> MTDRPDHIDSRVWELSETQEDWITQVHGHVRRVVECWKYTICCLISNMHTHRGAPQYDVFKWQDRSTIEWICSKKKVQYPERDTPDLYDNERAVAYKVLLVSDLSDHSPTSGIYHDLAFNLEGEAEESCALVLRGSQLQDIK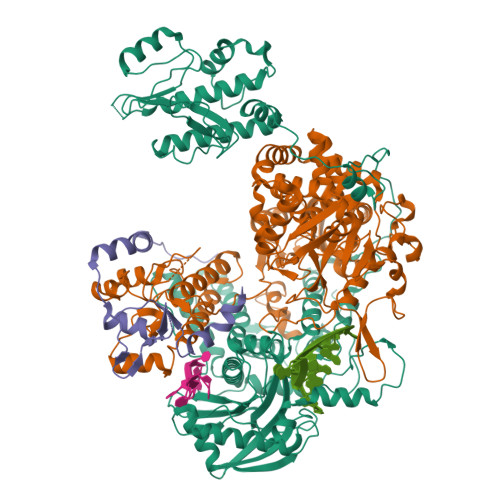GFLCRALEWVVSNNLTQEVVETISGEAKLQFSVGTTFRTLLKRDTDWDVIPTPRVEPNVPRIEGRRWTQMKKLPLLKEKEGPPSPWRALLLGADSEYIVCPPGTDQEAISWIHSQSEIECIRESKSTPASVITCLTSSLQSFAEGNPVRSRIHEDIIAFGINKKQEKKQSASSSASGEWKRAEYQVEEMSLPPWVEEEMVLLRSDQEDNWIELEKNAIYTEVDGVAEGLVDKYIEIVGRTKVASVIEKWQIAATRTFSQLHTDRSRITACPIITRDPSGNCQFWGMVLLGPHHVKRDTDNAPLLIAEIMGEDTEEKYPKHSVFSLKVEGKQFLLSLKITSFSRNKLYTFSNIRRVLIQPASIYSQVVLSRAAENNSLNLEVNPEIQLYLEGAQRGMTLYQWVRMILCLEFLMAIYNNPQMEGFLANMRRLHMSRHAMMERRQVFLPFGSRPEDKVNECIINNPIVAYLAKGWNSMPNVYY;> MNLFTPRSEINPTTTQELLYAYTGPAPVAYGTRTRAVLENIIRPYQYFYKEPNVQRALDIKTGCKEPEDINVEGPSSGFHTASVLKLADNFFRKYRPAMEKLKYWILVKLPKLKYAELSKGRQTYSFIHKRNLPAPIALEETVEFLEQNLRRKIGPTLLSYCQAIADVMELDETTYEGARDPRPWDIQLEEIDSDEEDPLFRQVGREETYTIKFSREELWDQMRTLNTMWKHLERGRLNRRTIATPSMLIRGFVKIVEDAAKEILENVPTSGVPVGGEEKLAKLASKQTFHTAVTGELSGDQEKFNECLDPDAMRLMWTVFLRKLGCPDWIMELFNIPFMVFKSKLADMGEGLVYTKGKLTDRKPLGEMPSEFDDLVRNVVGNSISCRLGMFMGMYNLTSTLLALISIEREELTGSHVESSDDFIHFFNCKTHEEMFKQAETLRLTLKLVGINMSPSKCILISPAGIGEFNSKFHHRDFVGNVATELPALVPNGTNPMTDLAMGLNVIKHSVNTGQMNLCTGALAMRIFNHAYKYAYMALGVTRRTRFMEENAITPLLTNQGASPVHSFSTMHLDEVALRRHLGLLDEETLRRILNPNNPVTQKGDPSMFFRIENKMPQIMEDYSVPSCFKYTLSRNRTIQDKPHKALLNKEERYQRVTSIINKLFPEVLIQEASAPGTVRESLKRRLELVVERSDLDEERKKRILSRIF;> MDREEPAESECTLRALVEEYNGACKEAPKEMSKQFTDYNTFKRYTTSKKDHAPQMRLVYSVRKPWPISMTPSKEIPLVFNGTKLKDTILDLGESKRTRANIVVPDYWSKYGSQTSLEVVNAILYAEDLKVQRFFSTEWGEIRYGRMLPFRKPVQACPTIEEVNPASIPHTLLQVFCPQYTTLDSKRKAHMGAVEKLKRVMEPICKVQTQESAVHIARSLIDSNKKWLPTVVDHTPRTAEMAHFLCSKYHYVHTNTQDLSDTRSIDNLCGELVKRSLKCRCPKETLVANLDKITIQGRPMREVLADHDGELPYLGICRVAMGLSTHHTMKIRSTKFSILNSDHPRIEVKKVFSLSPDVQVTIPYRRFKGKAKVYFQNDQIQGYFSCTDRQIDEIKISAPKNAPLLEPLLDICYYGSFIEPGFEQTFGFYPAGKREFVDSFFMHHSKDHKAFLIHMGLDKDLSLPLSPELNWKEPALSKVCRVTELDSTVQPYTSATREFVLGETLNVYTQHENGLELLICPTEIRSTRGPLPPGTNLSGSEFIDIYQDPFSRAKSLLKSTILHAERCKEFVGNMLEEYQDPAETTVQSLVPINTWGKSAKRKLQEEITSDPDWHQCPRKRAKMSYLAIIAGSIQDRDKKQTNVPRAFMLRGSQIEYDMKATRGLVVDTTNRIIVGGETVLREGKGGPEGYVQTGVFEEQPRCYLVDTPDHGLSMGLSRFCVHSQGRYFQYEKKISIWEETDNIKATIDSQRDLKRRRDIEEMVSKRARIV> GEGMWVPQQLPEIAGPLKKAGLKLSPQQISDLTGDPMGAVVALGGCTASFVSPNGLVVTNHACAYGAIQLNSTAENNLIKNGFNAPTTADEVSAGPNARVFVLDEITDVTKDAKAAIAAAGDDALARTKALEAFEKKLIADCEAEAGFRCRLYSFSGGNTYRLFKNLEIKDVRLAYAPPGSVGKFGGDIDNWMWPRHTGDFAFYRAYVGKDGKPAAFSKDNVPYQPKHWLKFADQPLGAGDFVMVAGYPGSTNRYALAAEFDNTAQWTYPTIARHYKNQIAMVEAAGKQNADIQVKYAATMAGWNNTSKNYDGQLEGFKRIDAAGQKLREEAAVLGWLKGQGAKGQPALDAHAKLLDLLEQSKATRDRDLTLALFNNTAMLGSATQLYRLSIEREKPNAERESGYQERDLPAIEGGLKQLERRYVAAMDRQLQEYWLNEYIKLPADQRVAAVDAWLGGNDAAAVKRALDRLAGTKLGSTEERLKWFAADRKAFEASNDPAIQYAVAVMPTLLKLEQERKTRAGENLAARPVYLQALADYKKSQGEFVYPDANLSLRITFGNVMGYAPKDGME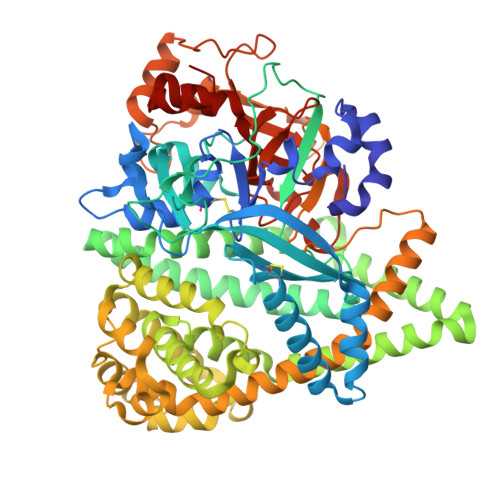YTPFTTLEGVVAKETGQDPFDSPKALLDAVAAKRYGGLEDKRIGSVPVNYLSDLDITGGNSGSPVLDAHGKLVGLAFDGNWESVSSNWVFDPKMTRMIAVDGRYLRWIMQEVYPAPQLLKEMNVGK> AQQGVFTLP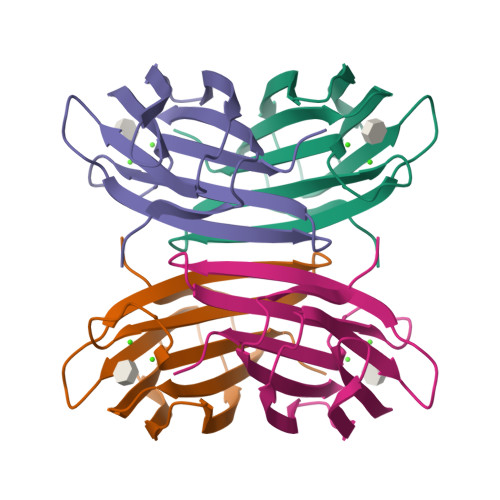ANTSFGVTAFANAANTQTIQVLVDNVVKATFTGSGTSDKLLGSQVLNSGSGAIKIQVSVNGKPSDLVSNQTILANKLNFAMVGSEDGTDNDYNDGIAVLNWPLG>MHHHHHHMPLEPHFMPDFLGHAENPLREEEWARLNETVIQVARRSLVGRRILDIYGPLGAGVQTVPYDEFQGVSPGAVDIVGEQETAMVFTDARKFKTIPIIYKDFLLHWRDIEAARTHNMPLDVSAAAGAAALCAQQEDELIFYGDARLGYEGLMTANGRLTVPLGDWTSPGGGFQAIVEA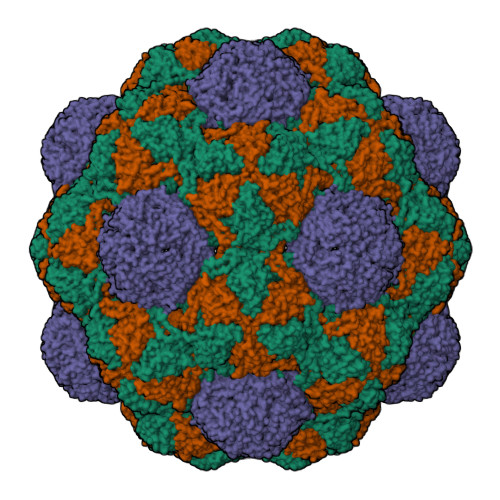TRKLNEQGHFGPYAVVLSPRLYSQLHRIYEKTGVLEIETIRQLASDGVYQSNRLRGESGVVVSTGRENMDLAVSMDMVAAYLGASRMNHPFRVLEALLLRIKHPDAICTLEGAGATERR[3x];>ESHPLTVGSLRR[3x]>[5x]HPETLVKVKDAEDQLGGRVGYIELDLASGKILESFRPEERFPMMSTFKVLLC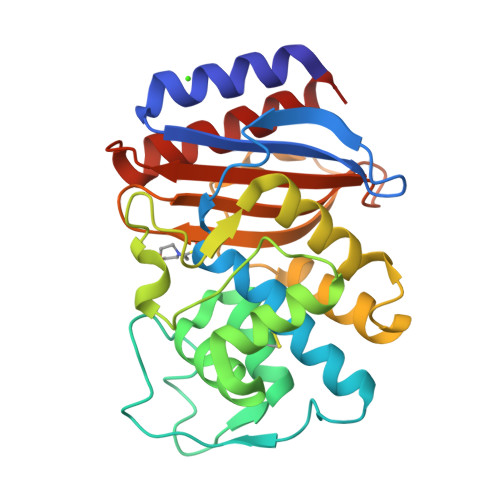GAVLSRVDAGQEQLGRRIHYSQNDLVEYSPVTEKHLTDGMTVGELCSAAITMSDNTAANLLLTTIGGPKELTAFLHNMGDHVTRLDRWEPELNEAIPNDERDTTTPVAMATTLRKLLTGELLTAASRQQLIDWMEADKVAGPLLRSALPAGWFIADKSGAGERGSRGIIAALGPDGKPSRIVVIYMTGSQATMDERNRQIAEIGASLIKHW>MSANDLPRGPEEGAPERKTREKPSQEQTDWSGSFSAYLESHRASLVDSLRRLFGHPFGSFFTCLVMGITLSLPMGLSLLLNNVERLGGSWQRAAQISLFLDLKTSENQGQDLREQIERLPDVIEAQLISREQALSELQEQSGLGEALKELPENPLPPVISVTPKQIDRAGLEALRQQLAELPHVQQAQLDLVWVERLSAILKLGERFVFGLTILLVLTLLLVVGNTIRLHIENRRNEIEVIKLVGGTDGYVRRPFLYMGALYGLGAGILSWALLAYSLNWLNGSVVNLSGLYGSDFGLQGVPLDDGLSLTVGAVLLGWVGAWLAVARHLRELAPR[2x];>[2x]MIRFEQVGKRYPNGHVGLHEVSFRVHRGEILFVTGHSGAGKSTLLRLILAMERPTSGKLLLGGQDLGRITTAQIPFLRRQIGVVFQNHQLLTDRTVADNIALPLQILGMPKPEIAKRVASALERVNLKEKGEALPSDLSTGQQQRVGIARAIVHQPALLLADEPTGNLDPRLASEIMGVFEDINRLGTTVLIASHDLALIARMRHRMLTLQRGRI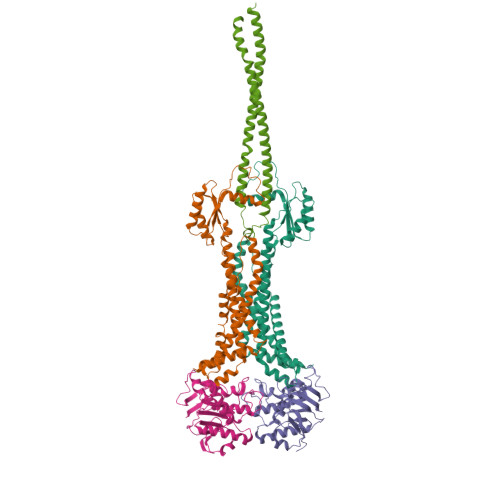IADREDEA;> DERADTQRQLEQTQKDIGELKKLLDGIQQEKSGVQKQLKSTETEMGDLEKQIKALQDELDKSEAELKRLDGEKKKLQDARIEQQRLLAIQARAAYQSGREEYLKLLLNQEHPEKFSRTLTYYDYINKARLEQLASFNETLRQLANVEQDISAQKAEQLSKQGELDSRREALAATRKERQQALAKLNSDYRERDQKLKSRQQDQAELAKVLRTIEETLARQAREAAAAAERERQRALAAERERARQQQAAPGRVTSPPREPAPGPLVSSTGAVYGGAFGSARGKLPWPVNGRVVARFGSQRGDDPRAKWDGVLISASAGSTVRAVHGGRVVFADWLRGAGLLVILDHGGGYLSLYGHNQSLLKDAGDTVKAGDPIATVGTSGGQSSPAVYFAIRHQGRPADPTTWCRAQG(~{E})-3-[3-(dihydroxyboranyl)phenyl]prop-2-enoic acid | C9 H9 B O4 | 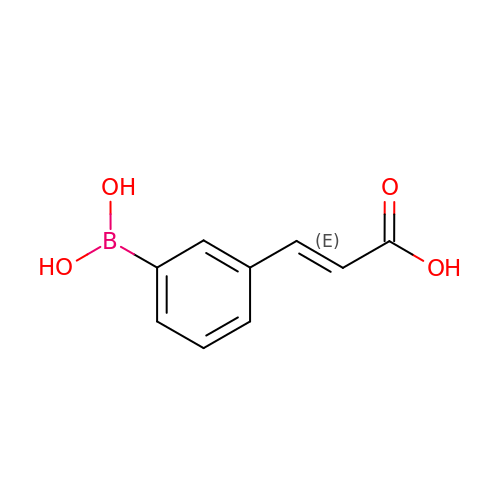QCHIEOGZUMAQKI-SNAWJCMRSA-N>[2x]EMCEIPEMDSHLVEKLGQHLLPWMDRLSLE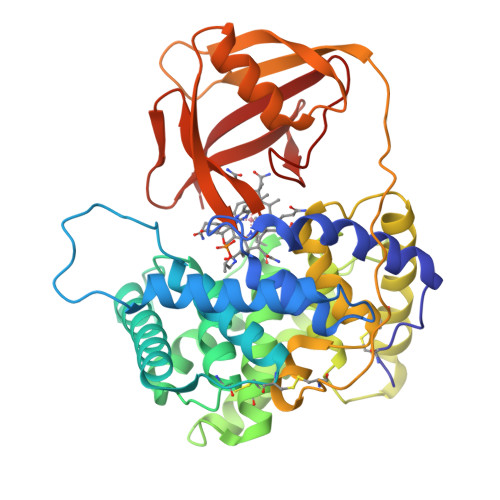HLNPSIYVGLRLSSLQAGTKEDLYLHSLKLGYQQCLLGSAFSEDDGDCQGKPSMGQLALYLLALRANCEFVRGHKGDRLVSQLKWFLEDEKRAIGHDHKGHPHTSYYQYGLGILALCLHQKRVHDSVVDKLLYAVEPFHQGHHSVDTAAMAGLAFTCLKRSNFNPGRRQRITMAIRTVREEILKAQTPEGHFGNVYSTPLALQFLMTSPMPGAELGTACLKARVALLASLQDGAFQNALMISQLLPVLNHKTYIDLIFPDCLAPRVMLEPAAETIPQTQEIISVTLQVLSLLPPYRQSISVLAGSTVEDVLKKAHELGGFTYETQASLSGPYLTSVMGKAAGEREFWQLLRDPNTPLLQGIADYRPKDGETIELRLVSW> ETGQTLAANIWSDKTTAQNEPINLTNANAPIKNAKNLNSTITNVAAFDTKLNHLLVDTITGRVFVGGVNRLYQLSPDLELSETVKTGPQNDSVECSILDCPLNAVRSPTDNYNKVLLIDRATSRLIACGSLFQGTCTVRNLQNVSIIEHEVPDAVVANDANSSTVAF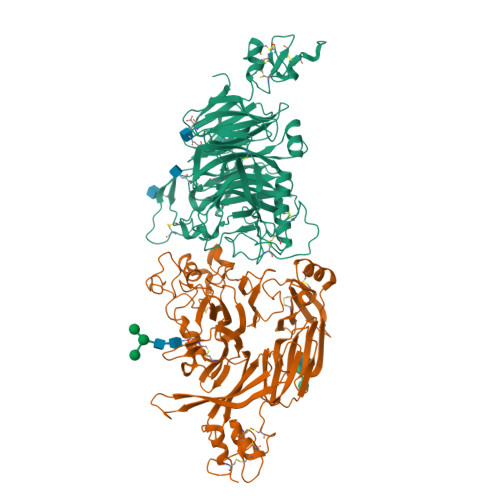IAPGPPQHPVTNVMYVGVTYTNNSPYRSEIPAVASRSLEKTKMFQIASSAVTTGTRTFINSYARETYFVNYVYGFSSERFSYFLTTQLKHSHHSSPKEYITKLVRICQEDSNYYSYTEIPVECISDAQGGTKFNLVQAGFLGKPSSDLAQSLGISIQDDVLFAVFSKGEGNTPTNNSALCIYSLKSIRRKFMQNIKSCFNGSGMRGLDFISPSMPCVLTKLQTIGEDFCGLDVNSPLGGETPITSVPVAMFNTKLTSVAATSTSGYTVVFVGTSDGFLKKVVIESSSIANEYASFAVDLGSEINRDMQFDNQNLYIYVMSKTKVSKVKVFDCSDYKTCGDCLGARDPYCGWCSLENKCSPRSNCQDDANDPLYWVSYKTGKCTTITSVVPHQLQRTTARTLELIIDHLPQLKENLICAFTTEDKALFTNATKKRNGVNCTTPRTDMLPQIEQGKHHFTAKLSVRTRNGPDLVSTDFTFFDCSTHSSCTRCVSSEFPCDWCVEAHRCTHDTAENCRNDILVTGVSRIGPSYRSGPGFCPTGTKHHHHHH;> ETGDVKPDLQTKQDKVLAHFIGNSTDYFKILDHNDEFVLVGAKDVIYNVSLNGLKEIARLEWHSTDADRELCALKGKHEWDCHNYLRVYALRPNGEVLLCGTNSYKPRCRHYTPVEVSSEEAGSAGHAHAMRYEVSRDVEAQGLCPYSPAHNSTYAFADGHLYSATVADFSGGDPLIYRENLRTEQYDLKQLNQPDFVGAIERNGYVLFFFRELSMEVMNFGKAVYSRVARVCKNDRGGPYSHGKSWTSFLKARLNCSVPGEFPFYFDEIQAISPIVESGSKSLIYAVFTTSVNAIPGSAVCAFNVDDILAAFDGEFKSQKDSQSHWLPVEREQVPKPRPGQCVEDSRTLTSIAVNFIKNHPLMEEAVPAVHGRPLLTKVNLHHRLTAIAVHPQVKSLSGAYYDVIYSGTDDGKVTKFINILSTHPNSTVDRLKTVVISEMQVLPLGTPIRELVISTSKNSLVVVSDGSLVSVPLHHCSHIVDCLGCLSLQDPICAWDLQTHECKNLATSQHKFGTKTYLQSLNSTKKAAALLCPHIPRDAPGAETVSFVTMAPPPTEEQKLLYSNVGSGTKHHHHHH>MSFDIAKYPTLALVDSTQELRLLPKESLPKLCDELRRYLLDSVSRSSGHFASGLGTVELTVALHYVYNTPFDQLIWDVGHQAYPHKILTGRRDKIGTIRQKGGLHPFPWRGESEYDVLSVGHSSTSISAGIGIAVAAEKEGKNRRTVCVIGDGAITAGMAFEAMNHAGDIRPDMLVILNDNEMSISENVGALNNHLAQLLSGKLYSSLREGGKKVFSGVPPIKELLKRTEEHIKGMVVPGTLFEELGFNYIGPVDGHDVLGLITTLKNMRDLKGPQFLHIMTKKGRGYEPAEKDPITFHAVPKFDPSSGCLPKSSGGLPSYSKIFGDWLCETAAKDNKLMAITPAMREGSGMVEFSRKFPDRYFDVAIAEQHAVTFAAGLAIGGYKPIVAIYSTFLQRAYDQVLHDVAIQKLPVLFAIDRAGIVGADGQTHQGAFDLSYLRCIPEMVIMTPSDENECRQMLYTGYHYNDGPSAVRYPRGNAVGVELTPLEKLPIGKGIVKRRGEKLAILNFGTLMPEAAKVAESLNATLVDMRFVKPLDEALILEMAASHEALVTVEENAIMGGAGSGVNEVLMAHRKPVPVLNIGL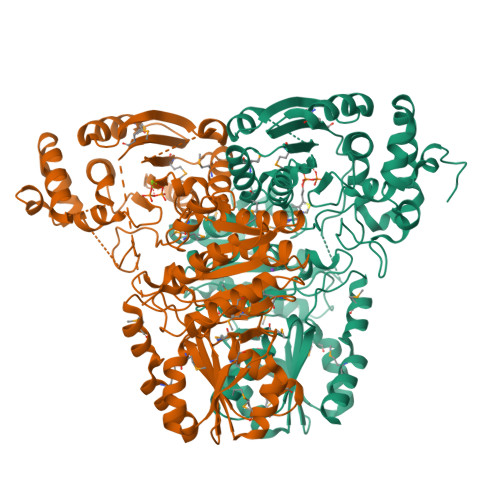PDFFIPQGTQEEMRAELGLDAAGMEAKIKAWLAL[4x]>GPPTSDDIFEREYKYGAHNYHPLPVALERGKGIYLWDVEGRKYFDFLSSYSAVNQGHCHPKIVNALKSQVDKLTLTSRAFYNNVLGEYEEYITKLFNYHKVLPMNTGVEAGETACKLARKWGYTVKGIQKYKAKIVFAAGNFWGRTLSAISSSTDPTSYDGFGPFMPGFDIIPYNDLPALERALQDPNVAAFMVEPIQGEAGVVVPDPGYLMGVRELCTRHQVLFIADEIQTGLARTGRWLAVDYENVRPDIVLLGKALSGGLYPVSAVLCDDDIMLTIKPGEHGSTYGGNPLGCRVAIAALEVLEEENLAENADKLGIILRNELMKLPSDVVTAVRGKGLLNAIVIKETKDWDAW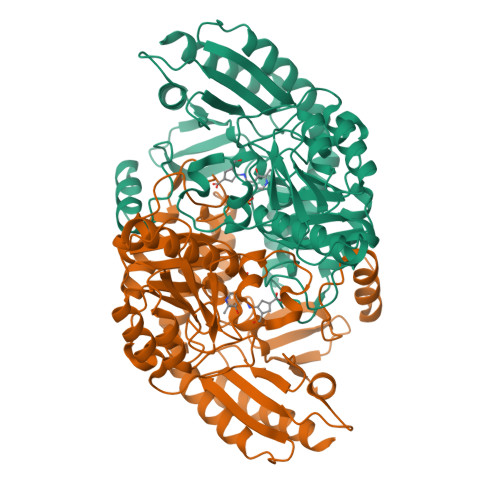KVCLRLRDNGLLAKPTHGDIIRFAPPLVIKEDELRESIEIINKTILSF[9x]>MKDLKKIESYLDKLRIKEKDGEERKIYAEVLDGRTLKTLYKLSAKGYITAMGGVISTGKEANVFYADGVFDGKPVAMAVKIYRIETSEFDKMDEYLYGDERFDMRRISPKEKVFIWTEKEFRNLERAKEAGVSVPQPYTYMKNVLLMEFIGEDELPAPTLVELGRELKELDVEGIFNDVVENVKRLYQEAELVHADLSEYNIMYIDKVYFIDMGQAVTLRHPMAESYLERDVRNIIRFFSKYGVKADFEEMLKEVKGE[2x]

Rio1 kinase is the founding member of the RIO family. Rio1 is involved in ribosome biogenesis, cell cycle progression and chromosome maintenance. Previously solved crystal structures of Archaeoglobus fulgidus Rio1 (afRio1) and Rio2 (afRio2) have shown the RIO domain is a trimmed version of the ePK catalytic domain with an additional conserved N-terminal α-helix. The afRio1 structure consists of an N-terminal domain (N-lobe) that consists of a α-helical region and a twisted β-sheet that contains the phosphate interacting loop (P-loop) and an α-helical C-terminal region (C-lobe) that houses the catalytic and metal binding residues.

We hereby present a crystal structure of toyocamycin bound to afRio1 at 2.0 Å resolution and employ structural analysis to characterize the interactions. The completely refined structure contained two molecules of the afRio1/toyocamycin complex per asymmetric unit with residues 3-258 for each molecule. The N- and C-lobes are connected by a hinge region, and between the two domains is a cleft that buries the 7-cyano-7-deazaadenine ring of toyocamycin. In the afRio1/toyocamycin complex, part of that flexible loop, residues 86–90 in chain A and residues 86–93 in chain B, are not observed in the electron density map. An overlay of the toyocamycin and ATP binding sites demonstrates that toyocamycin binds to the same site as ATP. Toyocamycin is buried in the active site pocket that features hydrophobic contact with Val 63, Ile 55 and Ala 78 from the N-lobe, Pro 156, Met 147,Phe 149 and Ile 150 from the hinge, and Met 203 and Ile 211 from the C-lobe. In addition, toyocamycin participates in ten hydrogen bond interactions. In the structure of the toyocamycin complex, the largest interface (836.5 Å2 per molecule) is observed between the two molecules of the asymmetric unit. The largest interface for both the ATP (766.6 Å2) and ADP (768.4 Å2) bound structures is the one similar to the largest interface in the toyocamycin complex. This interface positions the helices of the C-terminal lobe of one molecule (monomer A) in contact with both the N- and C-lobes at the opening of the active site of the second molecule (monomer B), almost completely occluding that active site. Specifically, in the adenosine bound structure, the backbone carbonyl oxygen bond of Ile 211 is pointing into the ATP binding pocket, while in the ATP and toyocamycin bound structures, there is a peptide flip that positions the Ile 211 carbonyl oxygen bond in the opposite direction, resulting in a 3.8 Å shift in position of the carbonyl oxygen.> MAKELSVYGPTAGESMGGTGANLNQQGGNNNSNSGVHWGGGSGSGNGGREHGSQTGWGWSKTNNPDVPPYVDDNGQVRITITNGLVKTPVYGVPGAGGNSDVQGGYIPENPNDEVARKWDKNNLPREIDVSIDGFKYRVTLNDNGRAIGILRTGVRPYVGSEKAKAGIMEKINHKTPEEIYEALGFNKDESQRQEKAKQQAEDAWDRLPPNVRKFDVDVEQFHYLVVLDDYGNVLSVTRTGVRPYVGSEKAKAGIMDKVDHKTPEEIYEALGFNNEEPQRQNQAKKAAYDVFYSFSMNRDRIQSDVLNKAAEVISDIGNKVGDYLGDAYKSLAREIADDVKNFQGKTIRSYDDA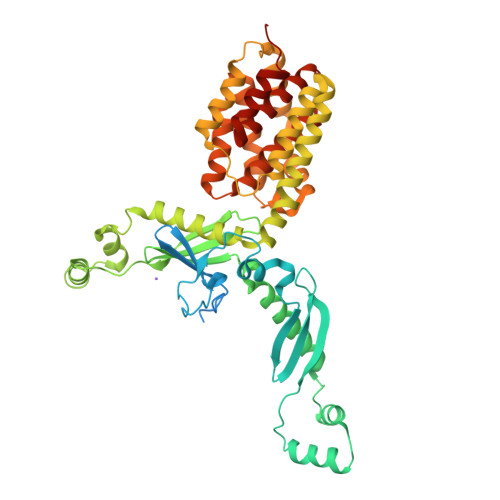MASLNKVLSNPGFKFNRADSDALANVWRSIDAQDMANKLGNISKAFKFADVVMKVEKVREKSIEGYETGNWGPLMLEVESWVLSGIASAVALGVFSATLGAYALSLGAPAIAVGIVGILLAAVVGALLDDKFADALNKEIIKPAHHHHHHH>FNVDNSGKGNCLYYAYSISLMYYLRAKNNVKITEDIFNKLGLKEEDRARLRKLLSKDPDRAFTRDEIKTIIEPILGRATRDLAAEHTKVEFKSSPHDTPLFSSLHYAVEFGFKRSLQINESELTLLIDNDFSNPDYTEAEIYKVSGLLDALQEYILTRTPSVIEEFNRQWENKKQELKEQSLTEKEIQVHQATILDNILRKETIDFLLAENEKHLDEYREHLRR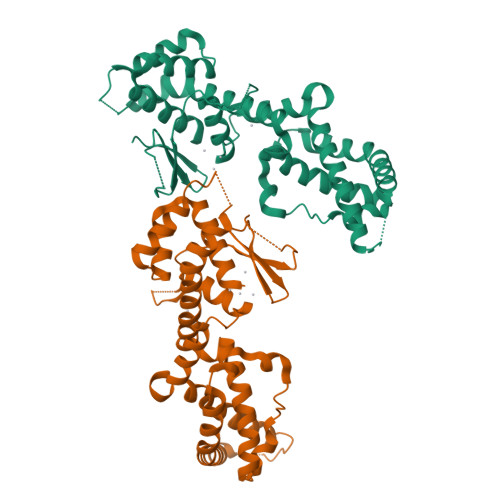EFVWGSEETLMVLHRAIQGERMVRNHEGRIEPVYDHEIILHVHRNGASPSYQAGSPEMILNNEGNVHWTSIIP[2x]> GPLGSMGKKSRVKTQKSGTGATATVSPKEILNLTSELLQKCSSPAPGPGKEWEEYVQIRTLVEKIRKKQKGLSVTFDGKREDYFPDLMKWASENGASVEGFEMVNFKEEGFGLRATRDIKAEELFLWVPRKLLMTVESAKNSVLGPLYSQDRILQAMGNIALAFHLLCERASPNSFWQPYIQTLPSEYDTPLYFEEDEVRYLQSTQAIHDVFSQYKNTARQYAYFYKVIQTHPHANKLPLKDSFTYEDYRWAVSSVMT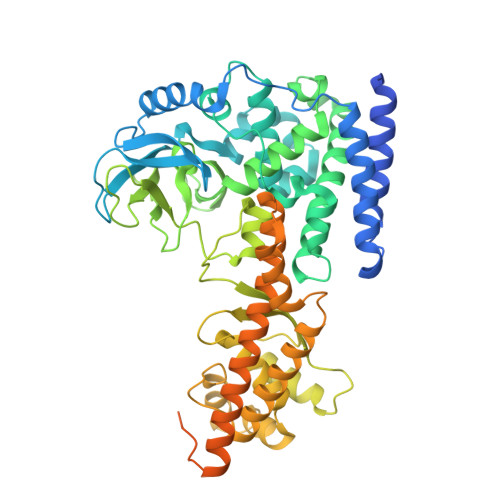RQAQIPTEDGSRVTLALIPLWDMCNHTNGLITTGYNLEDDRCECVALQDFRAGEQIYIFYGTRSNAEFVIHSGFFFDNNSHDRVKIKLGVSKSDRLYAMKAEVLARAGIPTSSVFALHFTEPPISAQLLAFLRVFCMTEEELKEHLLGDSAIDRIFTLGNSEFPVSWDNEVKLWTFLEDRASLLLKTYKTTIEEDKSVLKNHDLSVRAKMAIKLRLGEKEILEKAVKSAAVNREYYRQQMEEKAPLPKYEESNLGLLESSVGDSRLPLVLRNLEEEAGVQDALNIREAISKAKATENGLVNGENSIPNGTRSENESLNQESKRAVEDAKGSSSDSTAGVKE> MPLLVEGRRVRLPQSAGDLVRAHPPLEERARLLRGQSVQQVGPQGLLYVQQRELAVTSPKDGSISILGSDDATTSHIVVLRHTGNGATCLTHCDGTDTKAEVPLIMNSIKSFSDHAQCGRLEVHLVGGFSDDRQLSQKLTHQLLSEFDRQEDDIHLVTLCVTELNDREENENHFPVIYGIAVNIKTAEIYRASFQDRGPEEQLRA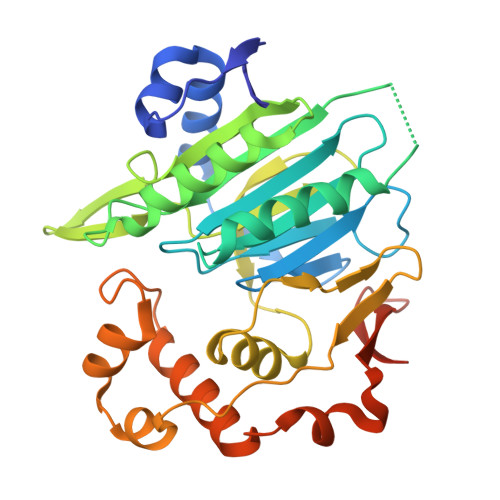ARTLAGGPMISIYDAETEQLRIGPYSWTPFPHVDFWLHQDDKQILENLSTSPLAEPPHFVEHIRSTLMFLKKHPSPAHTLFSGNKALLYKKNEDGLWEKISSPGSLEHHHHHH>MAQSSNSTHEPLEVLKEETVNRHRAIVSVMEELEAVDWYDQRVDASTDPELTAILAHNRDEEKEAAAMTLEWLRRNDAKWAEHLRTYLFTEGPITAANSSSVDKLAAALEHHHHHH[30x]

Our study reports on a new class of ferritin-like proteins (EncFtn), which are associated with bacterial encapsulin nanocompartments (Enc). By studying the EncFtn from R. rubrum we demonstrate that iron binding results in assembly of EncFtn decamers, which display a unique annular architecture. Biochemical assays show that EncFtn is active as a ferroxidase enzyme. While EncFtn does not store iron itself, its association with the encapsulin nanocage suggests that mineralization occurs within the cavity of the encapsulin shell (McHugh et al., 2014).

Through site-directed mutagenesis we show that the conserved glutamic acid and histidine residues in the FOC influence protein assembly and activity. Analysis of each of the single mutations (E32A, E62A and H65A) made in the FOC highlights the importance of the iron-coordinating residues in the catalytic activity of EncFtn.benzene-1,3-dicarboxylic acid | C8 H6 O4 | 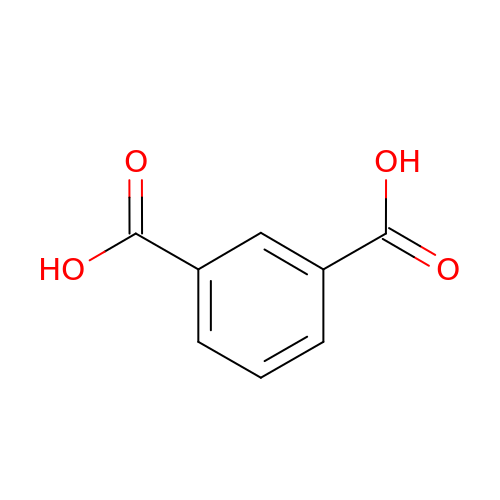QQVIHTHCMHWDBS-UHFFFAOYSA-N>SETFQDKVNFFQRELRQVHMKRPHSKVTLKVSRHALLESSLKATRNFSISDWSKNFEVVFQDEEALDWGGPRREWFELICKALFDTTNQLFTRFSDNNQALVHPNPNRPAHLRLKMYEFAGRLVGKCL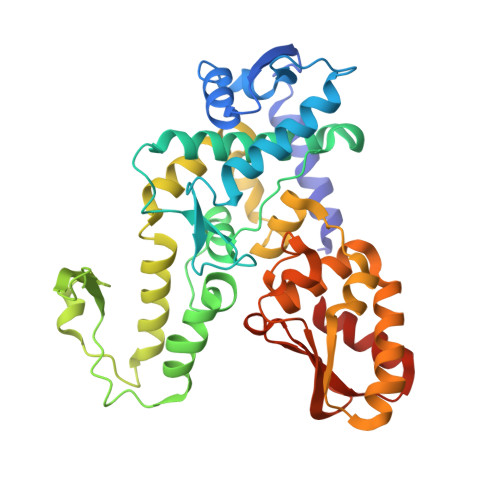YESSLGGAYKQLVRARFTRSFLAQIIGLRMHYKYFETDDPEFYKSKVCFILNNDMSEMELVFAEEKYNKSGQLDKVVELMTGGAQTPVTNANKIFYLNLLAQYRLASQVKEEVEHFLKGLNELVPENLLAIFDENELELLMCGTGDISVSDFKAHAVVVGGSWHFREKVMRWFWTVVSSLTQEELARLLQFTTGSSQLPPGGFAALCPSFQIIAAPTHSTLPTAHTCFNQLCLPTYDSYEEVHRMLQLAISEGCEGFGML[3x]>[4x]MGHHHHHQHMSTKQKLVGDVFSSVANRYDLMNDVMSLGIHRLWKDHFINKLDAGKRPNSTTPLNFIDVAGGSGDIAFGLLDHAESKFGDTESTMDIVDINPDMLKEGEKRAMEQGKYFKDPRVRFLVSNGEKLEEIDSDSKDIYTVSFGIRNFTDIQ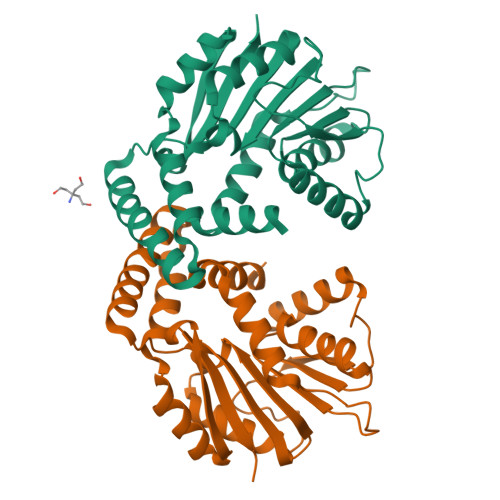KGLNTAYRVLKPGGIFYCLEFSKIENPLMDFAYQQWAKVLPVMGSMIANDYDSYQYLVESIERFPDQETFKSMIEKAGFKSAGYESLTFGICAIHWGIKV>MDDEDNKCDCPPPGLPLWMGTFANLMSLLMCFFVLLLSFS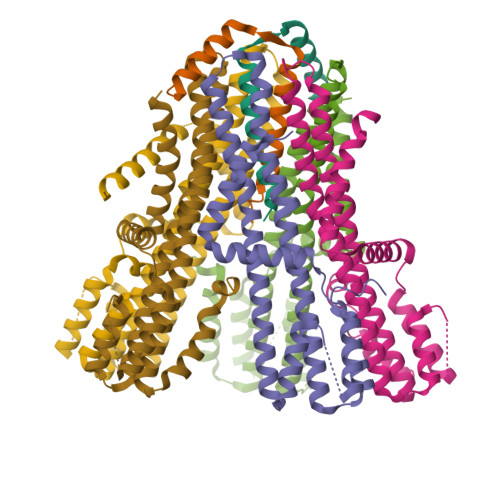EMDVLKFKQIAGSMKFAFGVQNQLEVKDIPKGTSIIAQEFRPGRPEPTPIDVIMQQTMDITQQTLEFHEGESDRAGGTKRDEGKLTGGQSPATSTQNNESAEADMQQQQSKEMSQEMETLMESIKKALEREIEQGAIEVENLGQQIVIRMREKGAFPEGSAFLQPKFRPLVRQIAELVKDVPGIVRVSGHTDNRPLDSELYRSNWDLSSQRAVSVAQEMEKVRGFSHQRLRVRGMADTEPLLPNDSDDNRALNRRVEISIMQGEPLYSEEVPVIQHHHHHH[2x];>[5x]MDLATLLGLIGGFAFVIMAMVLGGSIGMFVDVTSILIVVGGSIFVVLMKFTMGQFFGATKIAGKAFMFKADEPEDLIAKIVEMADAARKGGFLALEEMEINNTFMQKGIDLLVDGHDADVVRAALKKDIALTDERHTQGTGVFRAFGDVAPAMGMIGTLVGLVAMLSNMDDPKAIGPAMAVALLTTLYGAILSNMVFFPIADKLSLRRDQETLNRRLIMDGVLAIQDGQNPRVIDSYLKNYLNEGKRALEIDE The synaptic vesicle glycoprotein 2A (SV2A), a member of the major facilitator superfamily (MFS), is a key target for antiseizure medications and a biomarker for synaptic density imaging. SV2A is expressed in nearly all neurons, and mass spectrometry studies show that it is one of the most abundant membrane proteins in synaptic vesicles, with 5–12 copies present in each vesicle, indicating a function relevant to neurotransmission. Although its endogenous substrate and transport function remain elusive, SV2A is a target for clinical antiseizure drugs such as levetiracetam and brivaracetam. The transmembrane core adopts the canonical MFS fold, consisting of 12 transmembrane (TM) helices organized into two six-helix bundles, referred to as the N-domain and C-domain, connected by an intracellular segment that forms a long helix (ICH3).

We replaced 140 residues from the predicted disordered N-terminus of SV2A with a maltose-binding protein (MBP) tag (SV2AEM). We tested the function of SV2AEM by measuring the competition between unlabeled compounds and 3H-UCB-J. SV2AEM exhibited binding responses to levetiracetam, UCB-J, and padsevonil comparable to those of wild-type SV2A, indicating that the construct modification does not impair drug binding. We reconstituted purified SV2AEM protein into saposin nanoparticles and formed complexes with an MBP-specific DARPin30 to further increase the particle size for cryo-EM. We determined the structure of SV2AEM in the absence of ligands at 2.8 Å resolution. The transmembrane core and three short intracellular helices (ICH0–2) were well resolved. In contrast, the luminal domain was discernible in the 2D classification and unsharpened map, but lacked high-resolution features, likely due to its intrinsic flexibility. A central cavity lies at the interface between the N- and C-domains and is exposed to the luminal side of the synaptic vesicle, indicating that SV2A adopts a lumen-open conformation in the apo state, consistent with previous reports. However, we were unable to observe interpretable density for UCB1244283 in our cryo-EM reconstructions, and SV2A exhibited an apo conformation. This suggests that the allosteric site is not well formed in the unliganded SV2A, leading to low affinity for UCB1244283; orthosteric ligand binding induces formation of the allosteric site, resulting in increased affinity.

> AQRRKEREELAQQYEAILRECGHGRFQWTLYFVLGLALMADGVEVFVVGFVLPSAEKDMCLSDSNKGMLGLIVYLGMMVGAFLWGGLADRLGRRQCLLISLSVNSVFAFFSSFVQGYGTFLFCRLLSGVGIGGSIPIVFSYFSEFLAQEKRGEHLSWLCMFWMIGGVYAAAMAWAIIPHYGWSFQMGSAYQFHSWRVFVLVCAFPSVFAIGALTTQPESPRFFLENGKHDEAWMVLKQVHDTNMRAKGHPERVFSVTHIKTIHQEDELIEIQSDTGTWYQRWGVRALSLGGQVWGNFLSCFGPEYRRITLMMMGVWFTMSFSYYGLTVWFPDMIRHLQAVDYASRTKVFPGERVEHVTFNFTLENQIHRGGQYFNDKFIGLRLKSVSFEDSLFEECYFEDVTSSNTFFRNCTFINTVFYNTDLFEYKFVNSRLINSTFLHNKEGCPLDVTGTGEGAYMVYFVSFLGTLAVLPGNIVSALLMDKIGRLRMLAGSSVMSCVSCFFLSFGNSESAMIALLCLFGGVSIASWNALDVLTVELYPSDKRTTAFGFLNALCKLAAVLGISIFTSFVGITKAAPILFASAALALGSSLALKLPETRGQVLQ> MHHHHHHHAVRASEISRVYEAYPEKKATLYFLVLGFLALIVGSLFGPFQALNYGNVDAYPLLKRLLPFVQSYYQGLTLHGVLNAIVFTQLFAQAIMVYLPARELNMRPNMGLMWLSWWMAFIGLVVFALPLLANEATVLYTFYPPLKGHWAFYLGASVFVLSTWVSIYIVLDLWRRWKAANPGKVTPLVTYMAVVFWLMWFLASLGLVLEAVLFLLPWSFGLVEGVDPLVARTLFWWTGHPILYFWLLPAYAIIYTILPKQAGGKLVSDPMARLAFLLFLLLSTPVGFHHQFADPGIDPTWKMIHSVLTLFVAVPSLMTAFTVAASLEFAGRL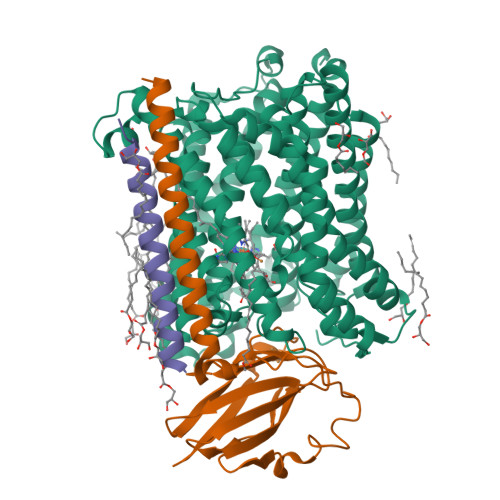RGGRGLFGWIRALPWDNPAFVAPVLGLLGFIPGGAGGIVNASFTLDYVVHNTAWVPGHFHLQVASLVTLTAMGSLYWLLPNLTGKPISDAQRRLGLAVVWLWFLGMMIMAVGLHWAGLLNVPRRAYIAQVPDAYPHAAVPMVFNVLAGIVLLVALLLFIYGLFSVLLSRERKPELAEAPLPFAEVISGPEDRRLVLAMDRIGFWFAVAAILVVLAYGPTLVQLFGHLNPVPGWRLW;> MVDEHKAHKAILAYEKGWLAFSLAMLFVFIALIAYTLATHTAGVIPAGKLERVDPTTVRQEGPWADPAQAVVQTGPNQYTVYVLAFAFGYQPNPIEVPQGAEIVFKITSPDVIHGFHVEGTNINVEVLPGEVSTVRYTFKRPGEYRIICNQYCGLGHQNMFGTIVVKE;> MEEKPKGALAVILVLTLTILVFWLGVYAVFFARG One function of Mediator complex subunit MED23 is to mediate transcriptional activation by the phosphorylated transcription factor Elk-1, in response to the Ras-MAPK signaling pathway. The MED23 subunit is the largest subunit of the Tail module and is specific to metazoans. The structure is composed of α-helices that engage in HEAT-repeat motifs, forming five solenoid regions which are designated as HR1 to HR5. The overall shape of MED23 is that of an arch with a concave and a convex face.

To validate the approach, we first determined the structure of MED23 alone by cryo-EM. We obtained a high-resolution structure of MED23, in which most of the structure is defined between 2.6-3 Å resolution, except for the N-terminal region, which appears more dynamic. The structure is comparable to the previously reported crystal structure40, with the main differences lying in the first N-terminal HEAT-repeat (residues 1–50), which appears dynamic. MED23 core is composed of HR2 to HR5 regions and adopts a triangular shape in which HR2 to HR5 coil to position the C-terminal HR5 region in close proximity to HR1, which protrudes out of MED23 core. We also observed that the 501-516 segment located at the HR2-HR3 junction is disordered in MED23Elk-1, whereas it is structured in MED23, where it folds into two short strands at the molecular surface. In MED23, this segment contacts HR4-lid and the HR2 region, in particular helix H19, and is therefore ideally positioned to detect allosteric changes resulting from Elk-1 binding. The closed HR4-lid region is not predicted to be a protein-protein interaction site in free MED23, whereas the region of MED23 exposed upon HR4-lid alteration has all the characteristics of a protein-protein interaction site. Overall the core of MED23 and MED23Elk-1 superimpose well for all HR regions (with mean rms deviations on Cα < ~ 0.6), except for the HR2 region, which appears slightly displaced upon binding of Elk-1.

> METQLQSIFEEVVKTEVIEEAFPGMFMDTPEDEKTKLISCLGAFRQFWGGLSQESHEQCIQWIVKFIHGQHSPKRISFLYDCLAMAVETGLLPPRLVCESLINSDTLEWERTQLWALTFKLVRKIIGGVDYKGVRDLLKVILEKILTIPNTVSSAVVQQLLAAREVIAYILERNACLLPAYFAVTEIRKLYPEGKLPHWLLGNLVSDFVDTFRPTARINSICGRCSLLPVVNNSGAICNSWKLDPATLRFPLKGLLPYDKDLFEPQTALLRYVLEQPYSRDMVCNMLGLNKQHKQRCPVLEDQLVDLVVYAMERSETEEKFDDGGTSQLLWQHLSSQLIFFVLFQFASFPHMVLSLHQKLAGRGLIKGRDHLMWVLLQFISGSIQKNALADFLPVMKLFDLLYPEKEYIPVPDINKPQSTHAFAMTCIWIHLNRKAQNDNSKLQIPIPHSLRLHHEFLQQSLRNKSLQMNDYKIALLCNAYSTNSECFTLPMGALVETIYGNGIMRIPLPGTNCMASGSITPLPMNLLDSLTVHAKMSLIHSIATRVIKLAHAKSSVALAPALVETYSRLLVYMEIESLGIKGFISQLLPTVFKSHAWGILHTLLEMFSYRMHHIQPHYRVQLLSHLHTLAAVAQTNQNQLHLCVESTALRLITALGSSEVQPQFTRFLSDPKTVLSAESEELNRALILTLARATHVTDFFTGSDSIQGTWCKDILQTIMSFTPHNWASHTLSCFPGPLQAFFKQNNVPQESRFNLKKNVEEEYRKWKSMSNENDIITHFSMQGSPPLFLCLLWKMLLETDHINQIGYRVLERIGARALVAHVRTFADFLVYEFSTSAGGQQLNKCIEILNDMVWKYNIVTLDRLILCLAMRSHEGNEAQVCYFIIQLLLLKPNDFRNRVSDFVKENSPEHWLQNDWHTKHMNYHKKYPEKLYFEGLAEQVDPPVQIQSPYLPIYFGNVCLRFLPVFDIVIHRFLELLPVSKSLETLLDHLGGLYKFHDRPVTYLYNTLHYYEMHLRDRAFLKRKLVHAIIGSLKDNRPQGWCLSDTYLKCAMNAREENPWVPDDTYYCRLIGRLVDTMAGKSPGPFPNCDWRFNEFPNPAAHALHVTCVELMALAVSGKEVGNALLNVVLKSQPLVPRENITAWMNAIGLIITALPEPYWIVLHDRIVSVISSPSLTSETEWVGYPFRLFDFTACHQSYSEMSCSYTLALAHAVWHHSSIGQLSLIPKFLTEVLLPIVKTEFQLLYVYHLVGPFLQRFQQERTRCMIEIGVAFYDMLLNVDQCSTHLNYMDPICDFLYHMKYMFTGDSVKEQVEKIICNLKPALKLRLRFITHISKMEPAAVPPQAMNSGSPAPQSNQVPVSLPVTQDVLFQGPGHHHHHH> MKVG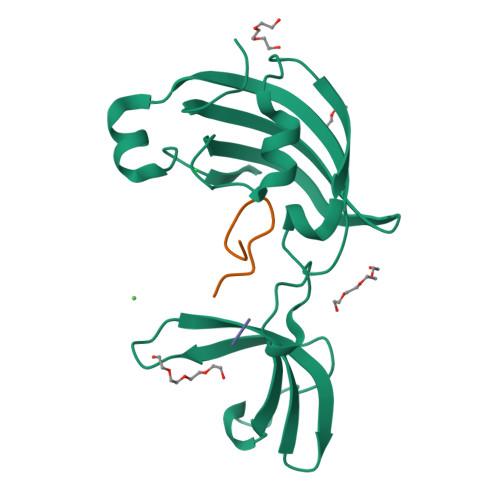QDKVVTIRYTLQVEGEVLDQGELSYLHGHRNLIPGLEEALEGREEGEAFQAHVPAEKAYGPHDPEGVQVVPLSAFPEDAEVVPGAQFYAQDMEGNPMPLTVVAVEGEEVTVDFNHPLAGKDLDFQVEVVKVREATPEELLHGHAHPSGHHHHHH;> TRYWNAKMLPFAFGA>[8x]GSMAGVIRLTPEELRGVARQYNVESSNVTELIARLDQMSHTLQGIWEGASSEA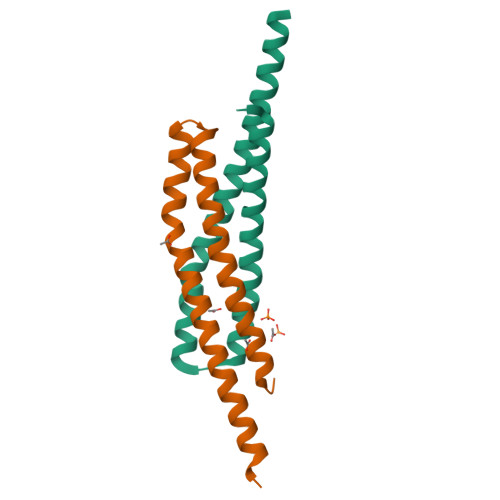FIQQYQELRPSFEKMAVLLNEVGQQLHNSATILEDTDQQIASQIRG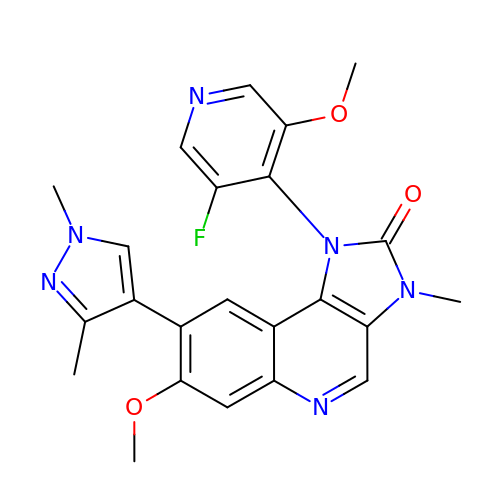8-(1,3-dimethylpyrazol-4-yl)-1-(3-fluoranyl-5-methoxy-pyridin-4-yl)-7-methoxy-3-methyl-imidazo[4,5-c]quinolin-2-one | C23 H21 F N6 O3 | WNEFOSMCGCLLJU-UHFFFAOYSA-N> GSHMTTSIKHAMGTTEIKGKPKRVVTLYQGATDVAVSLGVKPVGAVESWTQKPKFEYIKNDLKDTKIVGQEPAPNLEEISKLKPDLIVASKVRNEKVYDQLSKIAPTVSTDTVFKFKDTTKL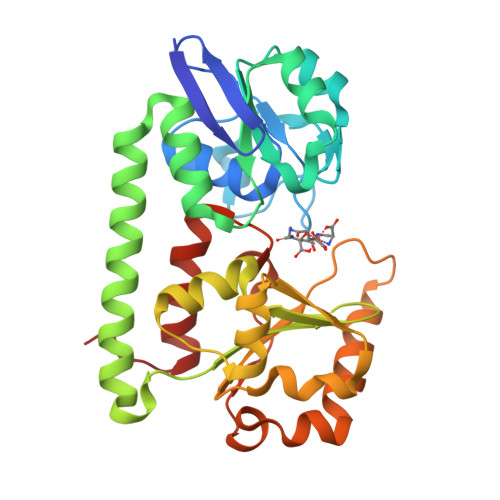MGKALGKEKEAEDLLKKYDDKVAAFQKDAKAKYKDAWPLKASVVNFRADHTRIYAGGYAGEILNDLGFKRNKDLQKQVDNGKDIIQLTSKESIPLMNADHIFVVKSDPNAKDAALVKKTESEWTSSKEWKNLDAVKNNQVSDDLDEITWNLAGGYKSSLKLIDDLYEKLNIEKQSK>[5x]MASLAAEPSDVFIGLKIDQITGIN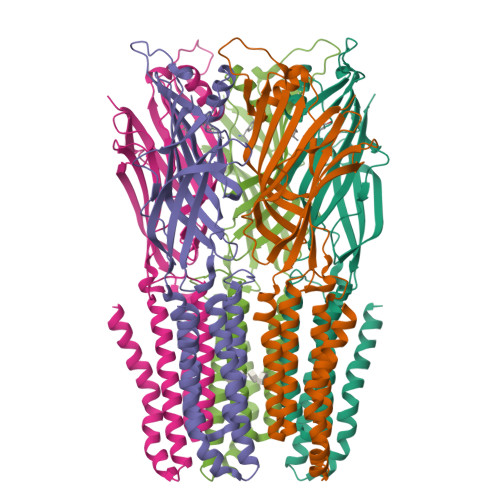QKEENFSVVGSLRIDWRQPLLAFEHAPGEPKHRTYTLATFLKLLEEKQIRWPAFTYHNQQGRMDFQNRLISLSEDGTVMYLERFTSTFQAPAFDFRLFPFDNQLFFIHVDSIFPQHLFRFQEMQGFSGLGDQLGEEEWIVTEVNTHLTTHNEFTKGDASRFVLEFHAERHLNYYLMRILIPVLLIITVSWFTFFLQDYTKRIDLAGGNLLLFIAFNFTISSDLPRLGYITLMDAFLVGTFIITALVVLGNVWLRRLENHGKQALARKLDIYAITSYPLAYLLGALTLWLLFFWRSY>[2x]MQDITMQWYQQLQDASMQCVLTFEGLTNSKDSQAKKIKMDLQKAATIPVSQISTIAGSKLKEIFDKIHSLLSGKPVQSGGRSVSVTLNPQGLDFVQYKLAEKFVKQGEEEVASHHEAAFPIAVVASGIWELHPRVGDLILAHLHKKCPYSVPFYPTFKEGMALEDYQRMLGYQVKDSKVEQQDNFLKRMSGMIRLYAAIIQLRWPYGNRQEIHPHGLNHGWRWLAQILNMEPLSDVTATLLFDFLEVCGNALMKQYQVQFWKMLILIKEDYFPRIEAITSSGQMGSFIRLKQFLEKCLQHKDIPVPKGFLTSSFWRS;>[2x]GPSGSIIATDNVLFTPRDKLTVEELEQFQSKKFTLGKIPLKPPPLELLN;>GPHMEDRAAQSLLNKLIRSNLVDNTNQVEVLQRDPNSPLYSVKSFEELRLKPQLLQGVYAMGFNRPSKIQENALPLMLAEPPQNLIAQSQSGTGKTAAFVLAMLSQVEPANKYPQCLCLSPTYELALQTGKVIEQMGKFYPELKLAYAVRGNKLERGQKISEQIVIGTPGTVLDWCSKLKFIDPKKIKVFVLDEADVMIATQGHQDQSIRIQRMLPRNCQMLLFSATFEDSVWKFAQKVVPDPNVIKLKREEETLDTIKQYYVLCSSRDEKFQALCNLYGAITIAQAMIFCHTRKTASWLAAELSKEGHQVALLSGEMMVEQRAAVIERFREGKEKVLVTTNVCARGIDVEQVSVVINFDLPVDKDGNPDNETYLHRIGRTGRFGKRGLAVNMVDSKHSMNILNRIQEHFNKKIERLDTDDLDEIEKIAN[2x]

At the cytoplasmic face of the NPC, Nxf1•Nxt1-bound mRNPs encounter the cytoplasmic filament nucleoporins Gle1, Nup42, and Nup214, which specifically activate the DEAD-box helicase DDX19 to remove Nxf1•Nxt1 from the mRNP8. DDX19 is a member of the DEAD-box helicase family, which are RNA-dependent ATPases composed of two RecA domains (referred to as DDX19NTD and DDX19CTD throughout the text). Gle1CTD plays an important organizational role by providing spatially separated binding sites for Nup42GBM and the DEAD-box helicase DDX19/scDbp5. A comprehensive structure-function analysis of DDX19 indicates that binding of Gle1CTD•Nup42GBM induces a conformational change in DDX19, thereby stimulating its ATPase activity.

To understand the structural basis for IP6-independent DDX19 activation, we determined crystal structures of human Gle1CTD•Nup42GBM in complex with DDX19 in the presence of ADP or AMP-PNP•Mg2+ at 3.6 and 3.4 Å resolution, respectively. The heterotrimeric Gle1CTD•Nup42GBM•DDX19∆N53 complex exhibited similar conformations in the presence of ADP or AMP-PNP•Mg2+, with the auto-inhibitory helix still bound between DDX19NTD and DDX19CTD. The inhibited state does not differ structurally in the presence of ADP or ATP, as the nucleotide-binding pocket readily accommodates the additional phosphate and Mg2+ ion, with minor changes in the sidechain conformations of K64 from the auto-inhibitory helix and E243 in the nucleotide binding pocket. The Gle1CTD−DDX19CTD interface involves 40 Gle1 and 35 DDX19 residues to generate an interaction interface area of almost 1300 Å2. In the structure of S. cerevisiae Gle1CTD•IP6•Dbp5∆N90(ADP), the interface between Gle1CTD and Dbp5CTD is only ~700 Å2 in surface area, compared to ~1300 Å2 for the human complex, a difference compensated for in yeast through extensive contacts made by both proteins with a bridging IP6 molecule. For a summary of differences, see Supplementary Note 4. These observed structural differences result in a dramatic reduction of the local electrostatic potential at the human Gle1CTD−DDX19CTD interface compared to the yeast Gle1CTD−DDX19CTD interface. Thus, for S. cerevisiae Dbp5 activation, the extreme negative charge of the IP6 molecule would be necessary to overcome the electrostatic repulsion generated in forming such a positively charged pocket, but for human DDX19 this requirement no longer exists. DDX19 is predominantly trapped in the auto-inhibited state, which can form in the presence of either ATP or ADP, although the ATP- and ADP-bound states could exhibit different dynamics for release of the auto-inhibitory helix. Gle1 binding facilitates release from auto-inhibition by first inducing conformational rearrangements in DDX19CTD that partially open DDX19 and generate a cleft between DDX19NTD and DDX19CTD (step 1).>GHKEVQLKDQILGVLDYLEKQQSAWPFLKPVSLSEAPDYYDIIKEPTDILTMRRKARHGDYKTKEDFGIELKRMFDNCRLYNAPTTIYFKYAN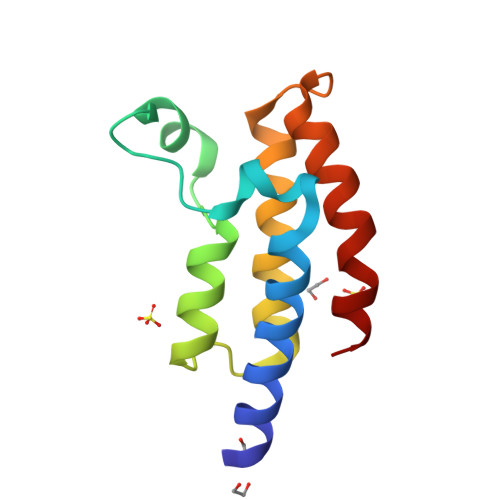ELQTLIWPKYEAI[4x]>[4x]SMDFMKPETVLDLANIRQALVRMEDTIVFDLIERSQFFSSPSVYEKNKYNIPNFDGTFLEWA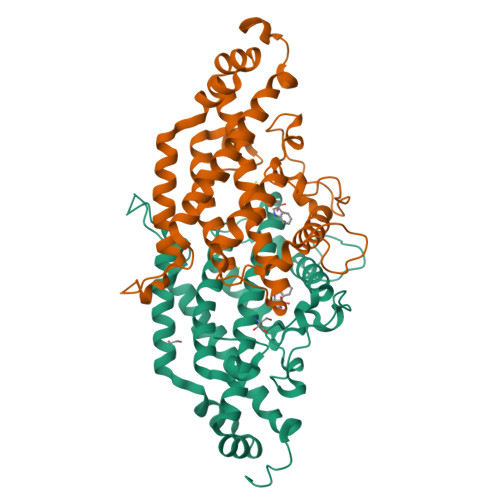LLQLEVAHSQIRRYEAPDETPFFPDQLKTPILPPINYPKILAKYSDEINVNSEIMKFYVDEIVPQVSCGQGDQKENLGSASTCDIECLQAISRRIHFGKFVAEAKYQSDKPLYIKLILDKDVKGIENSITNSAVEQKILERLIVKAESYGVDPSLKFGQNVQSKVKPEVIAKLYKDWIIPLTKKVEIDYLLRRLEDEDVELVEKYKK> TTCCPSIVARSNFNACRLPGTPEAL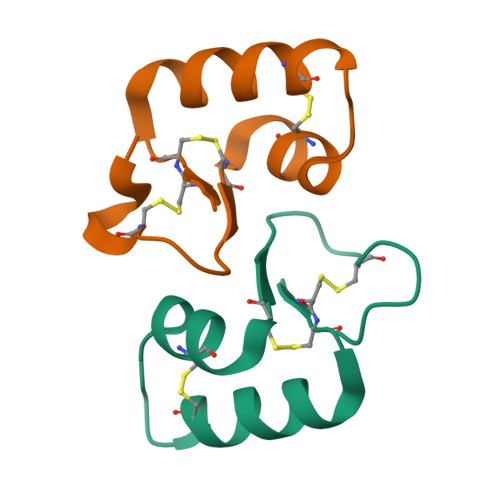CATYTGCIIIPGATCPGDYAN;> TTCCPSIVAKSNFNACRLPGTPEALCATYTGCIIIPGATCPGDYAN> MGSSHHHHHHSSENLYFQGHMKIGITCYPSMGGSGIIATELGIKLAERGHEVHFITS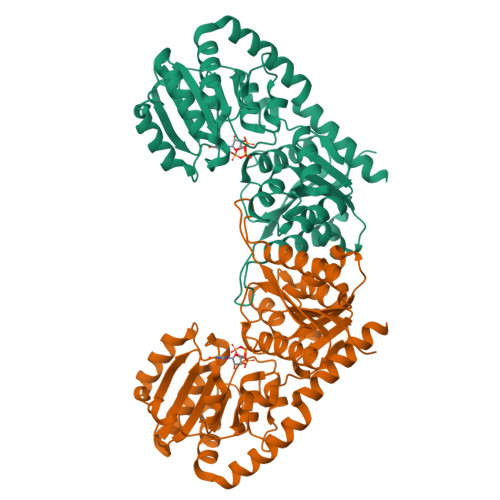NIPFRIRKPLPNMIFHQVEVNQYAVFQYPPYDITLSTKIAEVIKEYDLDLLHMHYAVPHAICGILAREMSGKDIKIMTTLHGTDITVLGYDHSLQGAIKFGIEKSDIVTSVSKSLAQETHEIIETNKEIIPIYNFVRENEFPTKHNTALKSQFGIAPDEKVLIHVSNFRQVKRIDTIIETFAKVREKIPSKLILLGDGPELVPMRQLTKELNVEEDVLFLGKQDCVSEFYQLSDLVLLLSEKESFGLTLLEAMKTGVVPIGSNAGGIKEVIKHGETGFVVDVGDCDSASDYAIRLLEDKVLYNKLQKNMLADIAERFGSELITDQYEYYYQKMLNEHNKSKGE Ub/Ubl protein conjugation can be reversed by specialized isopeptidases termed deubiquitinases (DUBs) or Ubl proteases, which antagonize Ub/Ubl-mediated post-translational modifications. Moreover, we focused on recently structurally characterized USPL1, which is the only deSUMOylase with a USP fold but for which its mechanism for SUMO paralogue specificity had remained unclear. USPL1 featured an approximately 25-fold higher activity for SUMO2 over SUMO1, which suggests a much more pronounced paralogue specificity as previously assumed from fluorogenic reagents. We structurally and biochemically explain this substrate selection, as USPL1 uses the USP fingers subdomain to contact the Gly27/Gly26 loop of SUMO2/3 to discriminate against SUMO1.

Taking inspiration from Ubiquitin- and ISG15-processing USP-substrate complexes, we semisynthetically obtained SUMO activity-based probes that contain a reactive warhead at the protein’s C-terminus. SUMO2 and SUMO3 feature identical Ubl folds and differ only in their unstructured N-terminal extensions. We prepared a SUMO3–2Br probe with a 2-bromoethyl warhead as well as a ΔN-SUMO2/3-PA probe equipped with a propargylamine warhead. Both probes reacted covalently with USPL1 as evident from a shift in molecular weight and led to pronounced protein stabilization as assessed by protein melting temperature analysis, indicative of the specific recognition of SUMO by USPL1. In contrast to a recently reported SUMO-dehydroalanine probe which reacted with USPL1 but not a SENP deSUMOylase, the ΔN-SUMO2/3-PA probe reacted with both USPL1 and SENP1, but not the DUB USP2. We solved crystal structures of USPL1 in covalent complex with ΔN-SUMO2/3-PA to 2.4 Å resolution, as well as of USPL1 in complex with SUMO3–2Br to 2.17 Å resolution in a different crystal form. Alignment of three independently obtained relative arrangements of the USPL1 and SUMO folds revealed near-identical positioning of SUMO in these highly conserved areas including the SUMO C-terminus, the Pro66 loop, as well as the Gly27 loop in the fingers. Recognition of the SUMO fold through the Gly27 loop is in striking contrast to Ubiquitin and ISG15 recognition by other USP enzymes which use a hydrophobic residue (Phe4 in Ub) as well as a large, complementarily shaped surface for many water-mediated interactions. In contrast, SENP1 cleaved all substrates completely, including the G27S mutant, which is not contacted by the SENP fold. These data demonstrate that the pronounced SUMO paralogue specificity of USPL1 toward SUMO2/3 over SUMO1 is based on USPL1’s ability to specifically recognize the Gly27 loop, as a serine at this position as in SUMO1 would disrupt the water-mediated interactions with USPL1.

> GPCTSFPQALCVQWKNAYALCWLDCILSALVHSEELKNTVTGLCSKEESIFWRLLTKYNQANTLLYTSQLSGVKDGDCKKLTSEIFAEIETCLNEVRDEIFISLQPQLRCTLGDMESPVFAFPLLLKLETHIEKLFLYSFSWDFECSQCGHQYQNRHMKSLVTFTNVIPEWHPLNAAHFGPCNNCNSKSQIRKMVLEKVSPIFMLHFVEGLPQNDLQHYAFHFEGCLYQITSVIQYRANNHFITWILDADGSWLECDDLKGPCSERHKKFEVPASEIHIVIWERKIS;> MINLKVAGQDGSVVQFKIKRHTPLSKLMKAYCERQGLSMRQIRFRFDGQPINETDTPAQLEMEDEDTIDVFQQQTG>[4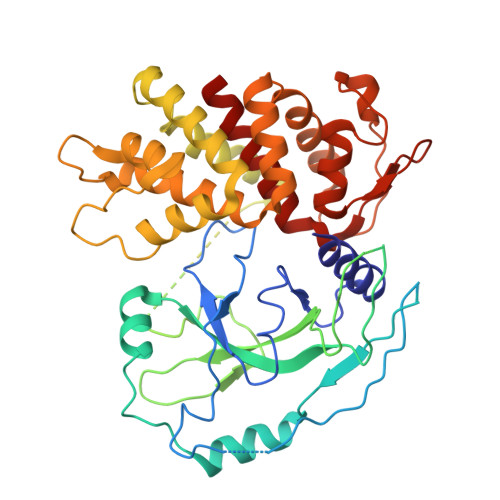x]SMGSAFERVVRRVVQELDHGGEFIPVTSLQSSTGFQPYCLVVRKPSSSWFWKPRYKCVNLSIKDILEPDAAEPDVQRGRSFHFYDAMDGQIQGSVELAAPGQAKIAGGAAVSDSSSTSMNVYSLSVDPNTWQTLLHERHLRQPEHKVLQQLRSRGDNVYVVTEVLQTQKEVEVTRTHKREGSGRFSLPGATCLQGEGQGHLSQKKTVTIPSGSTLAFRVAQLVIDSDLDVLLFPDKKQRTFQPPATGHKRSTSEGAWPQLPSGLSMMRCLHNFLTDGVPAELAFTEDFQGLRAEVETISKELELLDRELCQLLLEGLEGVLRDQLALRALEEALEQGQSLGPVEPLDGPAGAVLECLVLSSGMLVPELAIPVVYLLGALTMLSETQHKLLAEALESQTLLGPLELVGSLLEQSAPWQERSTMSLPPGLLGNSWGEGAPAWVLLDECGLELGEDTPHVCWEPQAQGRMCALYASLALLSGLSQEPH>GSHMKVEDPKDFPSELLSFLSHAVFSNRTLACFAIYTTKEKAALLYKKIMEKYSVTFISRHNSYNHNILFFLTPHRHRV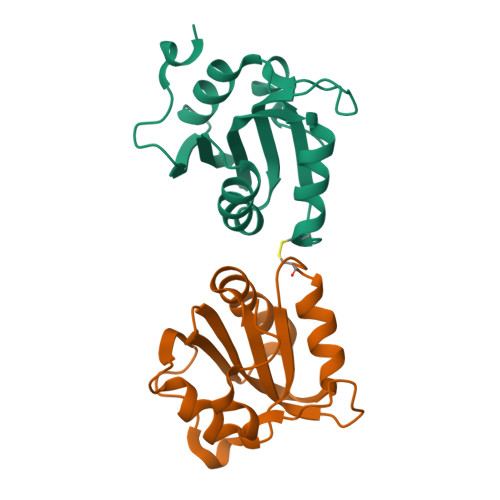SAINNYAQKLCTFSFLICKGVNKEYLMYSALTRDPFSVIEESLPGGLKEHDFNP[2x]> MSNITIYHNPACGTSRNTLEMIRNSGTEPTIILYLENPPSRDELVKLIADMGISVRALLKKNVEPYEQLGLAEDKFTDDQLIDFMLQHPILINRPIVVTPLGTRLCRPSEVVL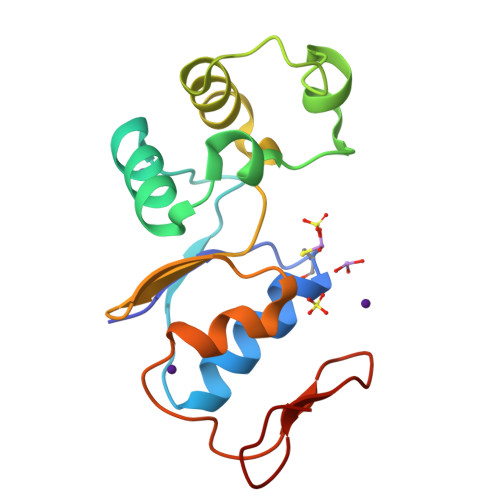DILQDAQKGAFTKEDGEKVVDEAGKRL> MHHHHHHNEIVVKGARVHNLKNITVRIPKNRLVVITGVSGSGKSSLAMDTIYAEGQRRYLESLSTYARQFLGNLKKPDVDEIEGLSPAIAIDQKT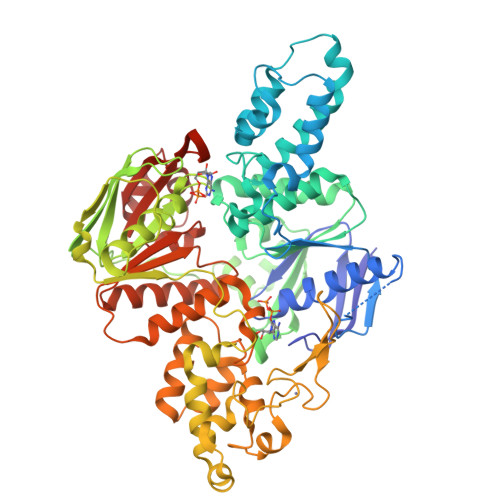VSHNPRSTVGTVTEIYDYLRVLYARIGKKINGLNIHEFTELSISEELEFLKNLNLTEREREIVGELLKEIEKRLEFLVDVGLEYLTLSRSATTLSGGESQRIRLATQIGSGLTGVIYVLDEPTIGLHPRDTERLIKTLKKLRDLGNTVIVVEHDEEVIRNADHIIDIGPGGGTNGGRVVFQGTVDELLKNPDSSLTGEYLSGKRKITVNKTRRLPYASLKIKGVRHNNLKNIDVEIPLGVFVCVTGVSGSGKSSLVMETLYPALMNLLHKTKLPAGEFDSIEGHENIDKMIAIDQSPIGRTPRSNPATYTKVFDEIRSLFAMTPAAKARGYNKSRFSFNLKGGRCEACQGQGYVKIEMLFLPDVYVECDVCKGKRYNRETLEITYKGKNISDILDMTVDEALEFFKNIPSIKRTLQVLHDVGLGYVKLGQPATTLSGGEAQRIKLASELRKRDTGRTLYILDEPTVGLHFEDVRKLVEVLHRLVDRGNTVIVIEHNLDVIKNADHIIDLGPEGGKEGGYIVATGTPEEIAKNPHSYTGRFLKNVL> KMAKLYMVSDASGSMRVTVVAEENPFSMAMLLSEECFILDHGAAKQIFVWKGKDANPQERKAAMKTAEEFLQQMNYSKNTQIQVLPEGGETPIFKQFFKDWRDK

Adseverin (also known as scinderin) is a member of the gelsolin superfamily of Ca2+-dependent actin-binding proteins, which regulate cytoskeletal dynamics by severing, bundling and capping of actin filaments. Adseverin is composed of six GH domains (A1–A6) and shares 60% overall sequence identity with gelsolin (G1–G6). Adseverin was first identified in chromaffin cells of bovine adrenal medulla, where it acts as an actin depolymerizing agent that disassembles the cortical network of actin filaments in response to bursts of intracellular calcium, leading to exocytosis of secretary vesicles. Crystallographic studies revealed that these binding events involve the association of eight calcium ions, six of which bind at a conserved site on each domain (type II), whereas the remaining two are also stabilized by contacts with actin (type I; refs 17, 18, 19, 20). Both proteins are able to sequester two monomers of actin, as well as sever and cap actin filaments through distinct Ca2+-induced domain rearrangements of the two halves of the molecule.

Unexpectedly, attempts to crystallize the active form of A1–A3 in the presence of 5 mM calcium led to a structure of Ca2+-bound A3 following protein degradation within the crystallization drop. Attempts to crystallize the active form of A1–A3 (aA1–A3) using a 5-mM CaCl2 supplemented protein sample led to the appearance of a single crystal after ∼80 days, from which a 1.8-Å data set was collected. The conformation of aA3 is highly similar to aG3, with a r.m.s.d. in Cα positions of 0.82 Å over 93 Cα atoms, and differs from inactive iA3 and iG3 by the position of the second β-strand and the straightening of the long α-helix. The structure is stabilized by Ca2+ coordination at the type II binding site, which involves interactions with Glu280 carbonyl, the carboxylates of Glu281 and Glu305, and three water molecules with bond distances ranging between 2.3 and 2.5 Å (inset). As previously noted for gelsolin, this Ca2+-bound conformation is incompatible with the formation of the A1–A3 latch, suggesting that calcium binding at A3 moves A1–A3 away from the inactive conformation through straightening of the A3 long helix resulting in the disruption of the A1:A3 interface. Furthermore, the structure of aA3 obtained by degradation of A1–A3 in the presence of calcium indicates that A3 may exist in a conformational state where it is distant from A1 and A2. The predominance of Int2 at high calcium concentration may explain the slow degradation of A1–A3 and crystallization of A3 in the presence of 5 mM calcium owing to the increased accessibility of the A1A2 and A2A3 linkers to proteolytic cleavage. This crystal structure revealed the presence of a single calcium ion bound at the type II binding site, associated with the straightened long α-helix that is characteristic of the active forms of gelsolin domains G3 and G6, highlighting the similarity of Ca2+-induced conformational changes in both proteins.> GLVLPHTEFQPAPKQDSSPHLTSQRPV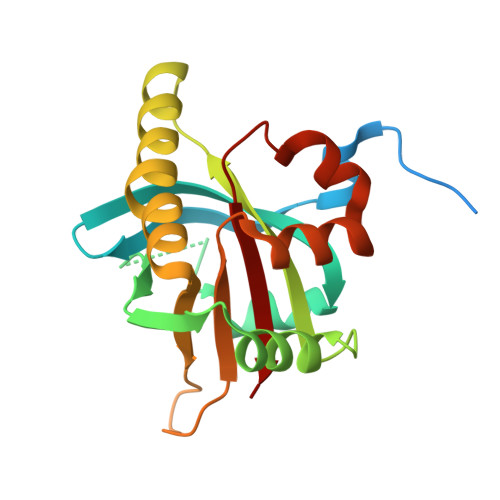DMVQLLKKYPIVWQGLLALKNDTAAVQLHFVSGNNVLAHRSLPLSEGGPPLRIAQRMRLEATQLEGVARRMTVETDYCLLLALPCGRDQEDVVSQTESLKAAFITYLQAKQAAGIINVPNPGSNQPAYVLQIFPPCEFSESHLSRLAPDLLASISNISPHLMIVIASV> LTFLEYW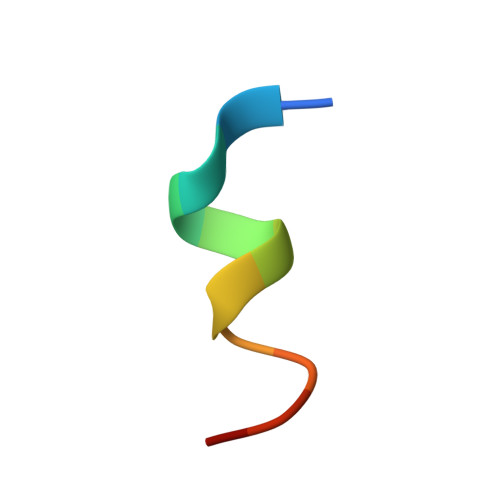AQLMQ> TPESVSELNHNHFLSPELQDKLDVMVSIYSCARNNNELEEIFQELSAFVSGLMDKRNSVFEVRNENTDEVVGALRAGMTIEDRDSYIRDLFFLHSLKVKIEESRQGK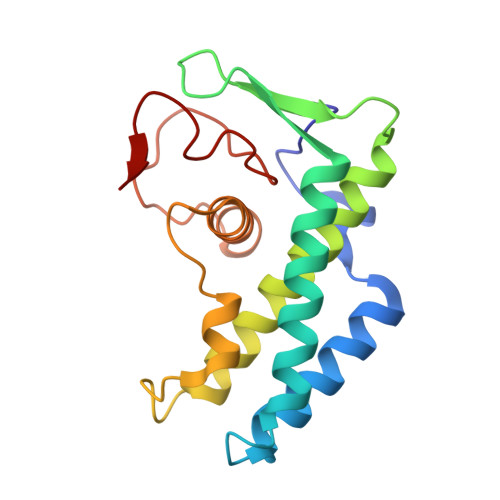EDSKCKVYNLLCPHHSSELYGDLRAMKCLVEGCSDDFNPFDIIRVPDLTYNKGSLQCG>[7x]GAMSEEKNLKTASVLSFERKLDPSDALFFSGNWSNKSDDKAWQPIHLREKSVRGTISNRLKKGEADPAKLNAAIEKPNLQTVDVATLPFDSDTLKVEFTLRVLGGVGEPAACNSMEYRSKLVATISHYIDTHGLDILGNRYAANLANGRFLWRNRLGADAISIQITRLSGDESTLVGVFDALAHPLRQFEEKSVSEELEALAKLITAGLAGQEHVLLRVKAFIRMGEGQEVFPSQELLLDKGKSTKSRFLYSVGQDEKAIAAIHSQKIGNALRTIDTWYPDAEINGPIAVEPYGSVTTQGVAYRQPKAKKDFYSLLDAWVLKDKEPTIEDQHFVAAVLVRGGVFGDAS

In the type I-F system, several Csy genes comprise a silencing Cascade complex with the Csy3 protein as a backbone-forming molecule. Among them, four genes of Csy1, -2, -3, and -4 (ZmCsy1-4) appear to form a silencing Cascade complex in the type I-F CRISPR systems. Based on the P. aeruginosa Cascade complex with a protein-helical backbone of six Csy3s, ZmCsy3 is predicted to form the molecular-helical backbone of the Z. mobilis Cascade complex. In order to provide a clue for the assembly mechanism of the Cascade silencing complex of the type I CRISPR/Cas system, the crystal structure of ZmCsy3 was determined.

There are seven ZmCsy3 molecules (ZmCsy3.1–ZmCsy3.7) in the asymmetric unit, and their structures superimpose very well onto each other, with a root-mean-square-deviation (rmsd) value of less than 0.2 Å. The monomeric ZmCsy3 structure is composed of ten α-helices (α1-α10) and eight β-strands (β1–β8) and forms a right-handed glove that is composed of a finger of several α-helices, a palm consisting of a β-sheet of 6 β-strands with an extended region (web), a thumb composed of a two-stranded β-sheet and an α-helix, and the backside of glove. The surface potential map reveals a positively charged surface patch within the glove and the inner sides of a finger and the thumb, and negatively charged surface patches on the backside of the glove and the outside of a finger and a thumb. The seven ZmCsy3 molecules in the asymmetric unit form an inter-molecular helical structure. At the inter-subunit interface, a thumb of one subunit interacts with a finger of the neighboring subunit, and the β-sheet of the five β-strands on the backside of one subunit comes into contact with those of the neighboring subunit(s) through many polar and hydrophilic interactions. In this oligomeric structure, the concave palms are twisted within a single molecule and form a continuous hollow cleft along the molecular helix, together with the extended regions (webs) and several loops in the fingers, and expose a long positively charged cleft to the solvent. The inter-molecular helix formed by seven ZmCsy3 molecules is part of a long superhelical filament structure in the entire crystal system, where seven molecules form a single turn with a diameter of ∼95 Å and a length of ∼82 Å. Since this molecular-helical structure is formed in the absence of crRNA in the crystalline state, there is a possibility that ZmCsy3 can be aggregated at high protein concentrations to form a molecular helical backbone of the Cascade effector complex without crRNA. The hexameric molecular-helix formed by ZmCsy3s, except for one ZmCsy3 subunit at either end in the apo-backbone structure, superimposes well onto the PaCsy3 helix backbone in the holo-Cascade structure, with rmsd values of less than 2.51 Å among the aligned 1912 Ca atoms, and only a negligible difference at the crRNA binding regions.5-FLUORO-1H-INDOLE-2-CARBOXYLIC ACID-(2-MERCAPTO-ETHYL)-AMIDE | C11 H11 F N2 O S | 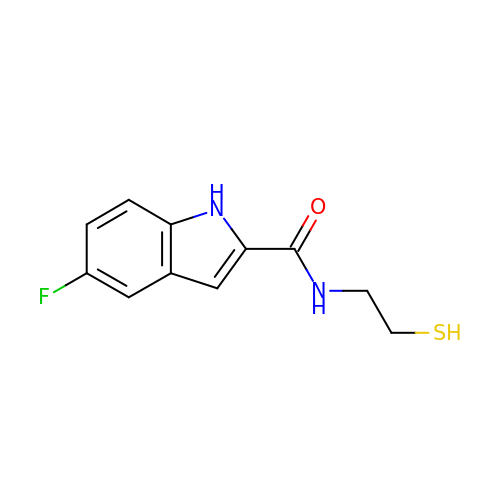JFUIHGAGFMFNRD-UHFFFAOYSA-N>MDLAKLGLKEVMPTKINLEGLVGDHAFSMEGVGEGNILEGTQEVKISVTKGAPLPFAFDIVSVAFTYGNRAYTGYPEEISDYFLQSFPEGFTYERNIRYQDGGTAIV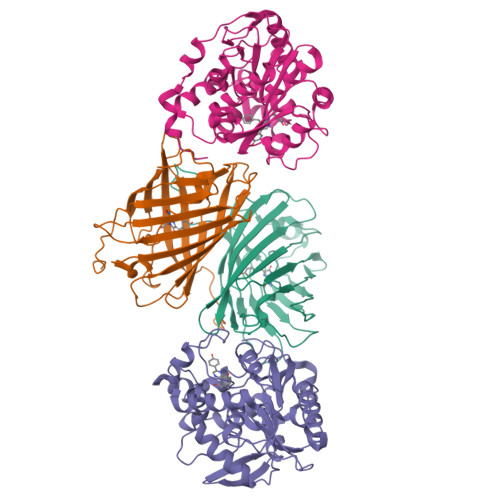KSDISLEDGKFIVNVDFKAKDLRRMGPVMQQDIVGMQPSYESMYTNVTSVIGECIIAFKLQTGKHFTYHMRTVYKSKKPVETMPLYHFIQHRLVKTNVDTASGYVVQHETAIAAHSTIKKIEGSLP[4x];>MTSKVYDPEQRKRMITGPQWWARCKQMNVLDSFINYYDSEKHAENAVIFLHGNATSSYLWRHVVPHIEPVARCIIPDLIGMGKSGKSGNGSYRLLDHYKYLTAWFELLNLPKKIIFVGHDWGAALAFHYAYEHQDRIKAIVHMESVVDVIESWDEWPDIEEDIALIKSEEGEKMVLENNFFVETVLPSKIMRKLEPEEFAAYLEPFKEKGEVRRPTLSWPREIPLVKGGKPDVVQIVRNYNAYLRASDDLPKLFIESDPGFFSNAIVEGAKKFPNTEFVKVKGLHFLQEDAPDEMGKYIKSFVERVLKNEQSGLEVLFQ[4x]> MAELQSGGGGGCCPPMDLFRSEPMQLVQIIIPIESAHLTVSYLGELGLLQFKD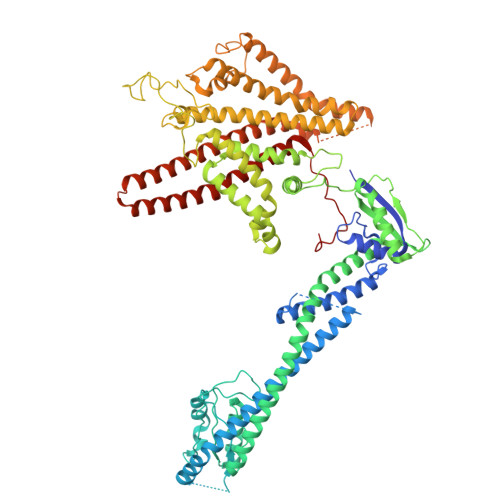LNSEKSPFQRTYAAQIKKCAEMARKLRFFKEQMLKAGILSSVKSTTRADNNTDDLEVKLGDLEAELVEINANGDKLQRAHSELVEYKLVLQKAGEFFSSALTSAAAQQREMESQQTGEMTIETPLLTDKEMSADPSKQIKLGFIAGLVPREKSMSFERMLFRATRGNVFLRQAVVDEPVVDPVSGEKMEKNVFVVFYSGERAKNKILKICDAFGANRYPFNEEFDKQAQAISEVSGRLSELKTTLDAGLLHRGNLLQTIGDQFEQWNLLVKREKSIYHTLNMLSLDVTKKCLVGEGWSPVFATKQIQDALERAAFDSNSQVGAIFQVLHTKESPPTYFRTNKFTSAFQEIVDAYGVAKYREANPGVFTIVTFPFLFAVMFGDWGHGICLLLGTLVLIVREKKLASQKLDDITDMTFGGRYVILMMALFSIYTGLIYNEFFSVPFEIFSHSAYACRDLSCSEATTVGLIKVRDTYPFGVDPVWHGSRSELPFLNSLKMKMSILLGVAQMNLGIILSYFNATFFRIGVNIWCQFIPQIIFLNSLFGYLSLLIILKWITGSQADLYHVMIYMFLSPTDELGDNQLFPGQKTAQLVLLLLAFVSVPWMLLPKPFILKMQHQDRHQGQSYEALQSTDESLQPDTNHDSHGHEEFEFSEVFVHQMIHTIEFVLGAVSNTASYLRLWALSLAHSELSSVFYEKVLLLAWGYNNILILIVGIIVFIFATVGVLLVMETLSAFLHALRLHWVEFQNKFYEGDGYKFSPFSFALLDDEDE The type II secretion system (T2SS) is a conserved transport pathway responsible for the secretion of a range of virulence factors by many pathogens, including Vibrio cholerae. In addition to cholera toxin, the T2SS in V. cholerae is responsible for the secretion of biofilm matrix proteins, chitin-binding and -degrading proteins, lipases, hemagglutinin/protease (HAP), a collagenase, and the serine proteases VesA, VesB, and VesC. Although many bacteria use the T2SS to support secretion of proteases, VesC is one of three unique trypsin-like serine proteases found in V. cholerae, other Vibrio species, and related marine species, including Aeromonas hydrophila, and may have a nonspecific and perhaps toxic activity inside the cell compared to other T2SS-secreted proteases. Analysis of VesC variants and the X-ray crystallographic structure of wild-type VesC suggested that all mutations lead to loss of VesC production and/or function.

Optimized crystals that diffracted to 2.2-Å resolution were produced from the construct pro-VesC containing residues 23 to 522, which includes the propeptide but not the N-terminal signal peptide or the C-terminal GlyGly-CTERM motif. The overall structure of VesC revealed that it consists of three domains: an N-terminal domain with a protease fold, the middle domain with an Ig-like domain, and the C-terminal domain with a β-sandwich fold. Well-defined electron density maps allowed the fitting of all three domains, the protease fold (35 to 272), the Ig-like fold (273 to 380), and the C-terminal domain (381 to 511), with the exception of the N-terminal residues (23–34), including the propeptide and C-terminal tail residues (512 to 522), due to their flexibility in the crystal structure. The structural comparison of the protease domain of VesC (VesCPD) with typical trypsins showed a high degree of structural similarity, with the best hit found in VesBPD. Consistent with the structures of VesBPD and other trypsinogens, VesCPD displays a similar positioning of its catalytic residues, and the three disordered loop regions (residues 164 to 172, 216 to 220, and 247 to 249) in the position of the active site are also observed in the crystal structure of VesCPD. In contrast, two loop regions, residues 115 to 121 and 194 to 208, in VesCPD adopt substantially different conformations, which extend upwards from the globular body of the protease domain. In the crystal structure, the interface between VesCPD and VesCIg buries a 1,568-Å2 solvent-accessible surface, which is ∼28% larger than the interface between the homologous domains in VesB. The structure of the third C-terminal domain of VesC, which is missing in VesB, revealed a concave β-sandwich domain. The high degree of structural similarity between VesCCBM and CBM family proteins suggests that VesC binds to carbohydrates and/or target glycosylated substrates.

> SGTESGVSSRIIGGEQATAGEWPYMVALTARNSSHVFCGGSYLGGRYVLTAAHCVDKEDPAKGDVLLGAFDMNDVNTAERIHVRQIYVHNSYITASMGNDIAVLELERDPLPRRSVQISDSSDFNELTKDSPMTVIGFGNRKEVDGEKSDPATILHQVQVPFVPLPECKTKGSDQDAKNNYSQLTNNAFCAGSFGKDACSGDAGGPIFFDSNNGRKQMGVVSWGDGCGRANSPGVYTNLSVFNDWLDDQQLGLSYRQKRDLGVVRPGSYTHNLTFTNNGNADINLGNTFVFVVGISRTDAAAIVNNSCTGVLASGASCDVEFSYNITEHKQSYVKLIIGSSTYKTGAVHAYLYFDALDAAPSETVSFLANLPVHNTHVNDHPWTVVGNGLQTSALPAGEESVILLENLPQGRLKFHYKLSSSEVLDQLFVYVNDKFKGKYFNNTENLATLDMYGTNNKVRFVYRRHSGSTDDQSRAILSQISYDPKFFDLPPPLDIRIGDENLYFQ> HMASKMFFINDETPWEELGNGIKRKVMTWSDDLMMVCVHFDKGAIG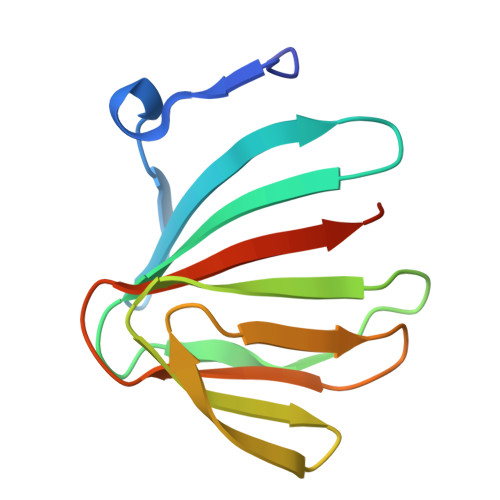VAHKHDIHDQIAYVAAGSFEVEIEGQKRILKAGDAYRAVKNEMHGAVSLEDNSILIDTFNPKRDDFL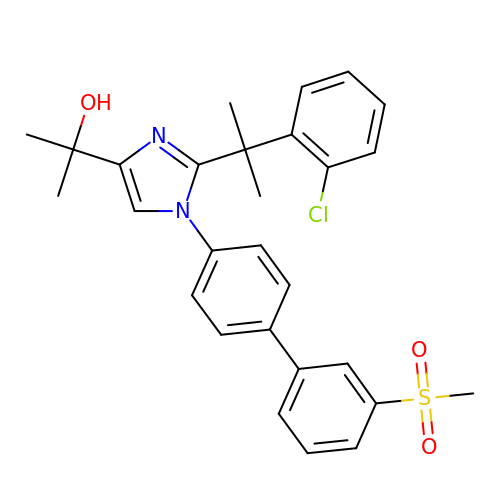2-{2-[2-(2-chlorophenyl)propan-2-yl]-1-[3'-(methylsulfonyl)biphenyl-4-yl]-1H-imidazol-4-yl}propan-2-ol | C28 H29 Cl N2 O3 S | JLPURTXCSILYLW-UHFFFAOYSA-N>[2x]GMCVEKTPWELVIDFH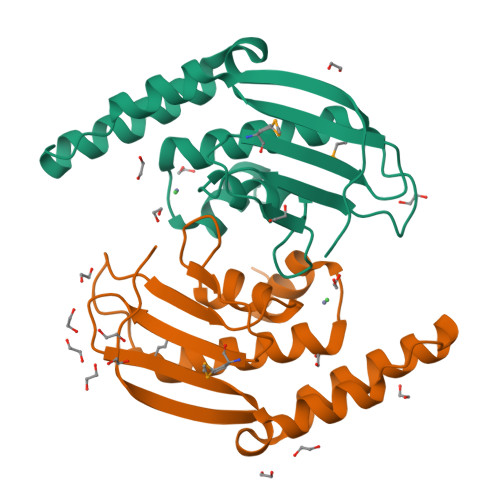GHTCPDIALGYRIAQLAQREMGIRPAPDSECLVKAYTQSCALDAIQVLNKATIGRHALIIEETHRYMYQFHFTGTQDIHQFTVSPAVLDHLETLRHPDLSPRERQNKVLEGVQYVLTLEESAFCHYDKIPGQLSKIV>[2x]MPLTDTDRSEDFLRRVRGLKAARTANGPRLYQPITLLWAVGRARRGEARTLAWADTDEAIGALLKRHGARGERPRP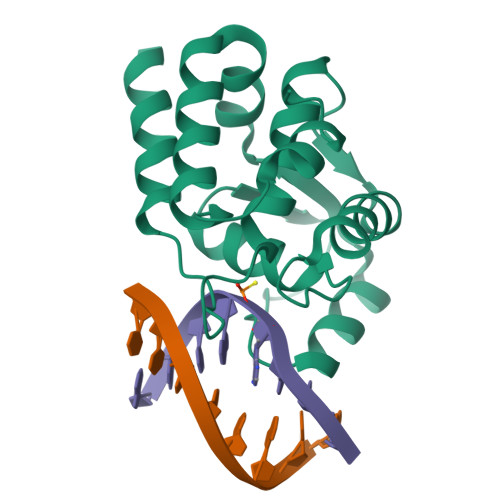DYPVLALHRAGLWTLEGHVGEVPTAHGDSALRNWFAEQRPVGGLAEPFHDLLHRSGHSRVSVIEALLTTYFAGLDPVPLLEDTGLYDEG> GS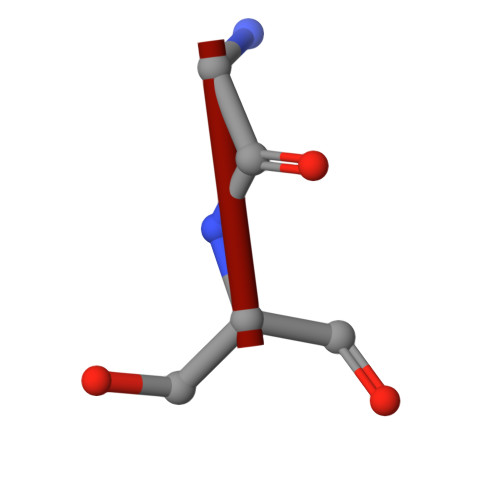GSGSGS>[20x]GSFTMADLDDIKDGKDFRTDQPQKNIPFTLKGCGALDWGMQSRLSRIFNPKTGKTVMLAFDHGYFQG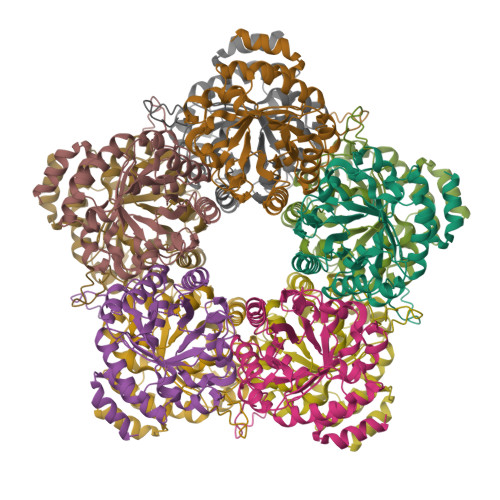PTTGLERIDINIAPLFEHADVLMCTRGILRSVVPPATNRPVVLRASGANSILAELSNEAVALSMDDAVRLNSCAVAAQVYIGSEYEHQSIKNIIQLVDAGMKVGMPTMAVTGVGKDMVRDQRYFSLATRIAAEMGAQIIKTYYVEKGFERIVAGCPVPIVIAGGKKLPEREALEMCWQAIDQGASGVDMGRNIFQSDHPVAMMKAVQAVVHHNETADRAYELYLSEKQ>GHMYAIAEDTLPARVLKELLLYRRRYPEHRQSASEADEIRRIEQVQLPRIAAFIEAGEPIEFVLPAFPAKSPNPGKVLDSRPDMAERLSLSFLNHL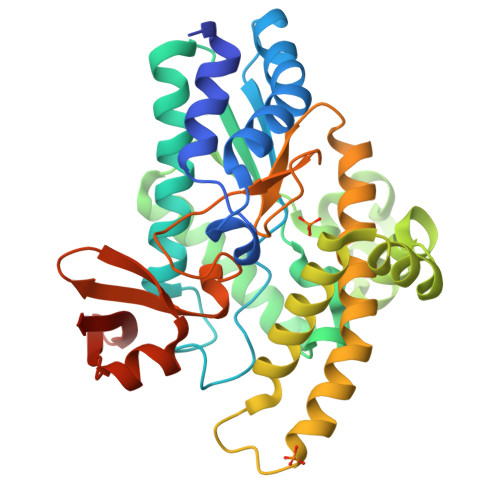CQRIQLFYAPGAKITVCSDGRVFGDLVRIGDAHISAYQDALRLMIEEIGATHIGVFNLEDVRAFEAQRDNHEQLRQLLIGGYAEPLESIRETLLASEEGLLLYRAITRFLYEDGLTPDYQGSKTALQRDAKERAYGVIQRSWAWGALLADQFPRAIRLSIHPQPADSLKFGIHMMPTRDDWLTPWHGVAVNTEDRFVLMKRSEVLELGGELVQINGQPSHYRLPARAARRAAVA[4x]> MTERTLKVLSPLHIGTGNELTPVDIYPRENIIHVLDTERLVNDLMNLGVELNEILALLKNPPGDAYIWKGYIEEFHLDPSDYSIYTLKIHGKIGRKSMQIKEFIKLNGRPYIPGSSLKGAIRTAVLYKALKECGDARAVMRVVSKVNGDVARDIGRSEDVLDYYMSFLSRARIDRKRADDLLEAIVFGMEPDRRSKIRYEPKRDPMKALIVRDSKPVGRKHLAVYHVEVIGNPQPIPIWV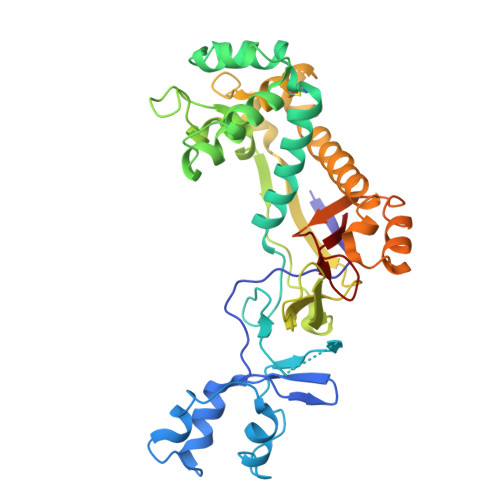EAIEPGAATDVEIHVDTEALRLNADYFNGLLWECLKERGEPGEVFEDFLWEAVDEFYTAVMKYETIEVQKFGRYTSQVRSFYASLEDHSGHVLRLGWGSGWLAMTIGLLLVEKGYKWENVRKKLGLGKKPGGSGFSREFPKTRRLADGMPMGWVVLE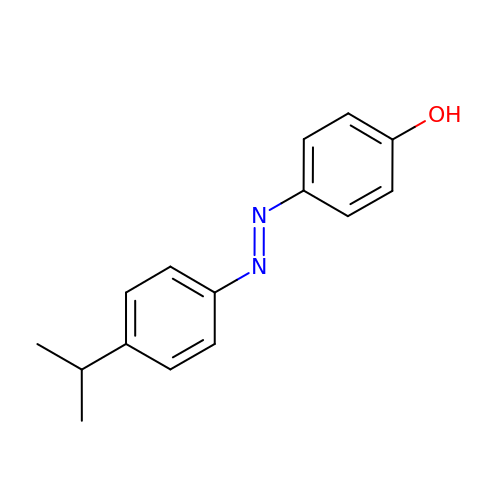4-{(E)-[4-(propan-2-yl)phenyl]diazenyl}phenol | C15 H16 N2 O | NQJVTPMZGHHWGR-WUKNDPDISA-N> MILNNQEWLLAIFKKKGLTPTGKLEFATIDGIDSALAQALNEAFDSQVVSFNDRINQSFREFLKRTPRDRITLGTFSDVKEWLSSFEADRAGRKDTASAGP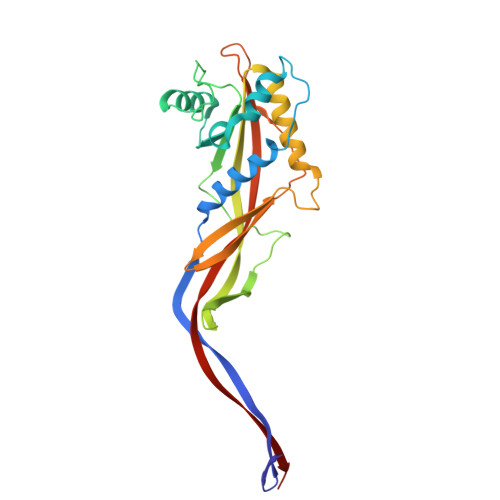VNKLAMPLVNLSRSPAFSIYEGELCRDNYDEGHVTNENDEIEALVSTIPFSLEYSLWIASDEKESLGMVTTALAFWLRMYASLGQASFTHIANVGGYEIPVTCYIEGQKSIAFQDLTTGTADNRLFAVGLNLTVVAELPILAYMQQTTGTITVKAKILEE>[26x]MQKYALHAYPVMALMVATLTGCAWIPAKPLVQGATTAQPIPGPVPVANGSIFQSAQPINYGYQPLFEDRRPRNIGDTLTIVLQENVSASKSSSANASRDGKTSFGFDTVPRYLQGLFGNSRADMEASGGNSFNGKGGANASNTFSGTLTVTVDQVLANGNLHVVGEKQIAINQGTEFIRFSGVVNPRTISGSNSVPSTQVADARIEYVGNGYINEAQNMGWLQRFFLNLSPM;>MFKALAGIVLALVATLAHAERIRDLTSVQGVRENSLIGYGLVVGLDGTGDQTTQTPFTTQTLNNMLSQLGITVPTGTNMQLKNVAAVMVTASYPPFARQGQTIDVVVSSMGNAKSLRGGTLLMTPLKGVDSQVYALAQGNILVGGAGASAGGSSVQVNQLNGGRITNGAIIERELPTQFGAGNTINLQLNDEDFTMAQQITDAINRARGYGSATALDARTVQVRVPSGNSSQVRFLADIQNMEVNVTPQDAKVVINSRTGSVVMNREVTLDSCAVAQGNLSVTVNRQLNVNQPNTPFGGGQTVVTPQTQIDLRQSGGSLQSVRSSANLNSVVRALNALGATPMDLMSILQSMQSAGCLRAKLEII[26x]

The bacterial flagellar motor is a huge bidirectional rotary nanomachine that drives rotation of the flagellum for bacterial motility. The cytoplasmic C ring of the flagellar motor functions as the switch complex for the rotational direction switching from counterclockwise to clockwise. The basal body is made up of the LP ring, MS ring, C ring, rod and export apparatus. Here, we present two high-resolution cryo-electron microscopy structures of the C ring-containing flagellar basal body–hook complex from Salmonella Typhimurium, which are in the default counterclockwise state and in a constitutively active CheY mutant-induced clockwise state, respectively.

Given the high fragility of the C ring, we examined several reagents as the media of density gradient centrifugation in the purification of the intact C ring-containing basal body–hook complex in the default CCW state from our previously constructed ΔfliCD strain of S. Typhimurium, which lacks the flagellar filament, thus avoiding effects of the filaments on purification of the motor. The cryo-EM density map of the C ring-containing basal body–hook complex in the default CCW state was successfully determined to an overall resolution of 7.4 Å. Local refinements of the LP ring, MS ring, rod, hook and export apparatus generated their high-quality cryo-EM density maps at the resolutions ranging from 3.0 Å to 4.3 Å. The LP ring acts as a bushing to stabilize the rotation of the rod, which serves as the drive shaft.>HHPMAETQTLLRNFGNVYDNPVLLDRSVTAPVTEGFNVVLASFQALYLQYQKHHFVVEGSEFYSLHEFFNESYNQVQDHIHEIGERLDGLGGVPV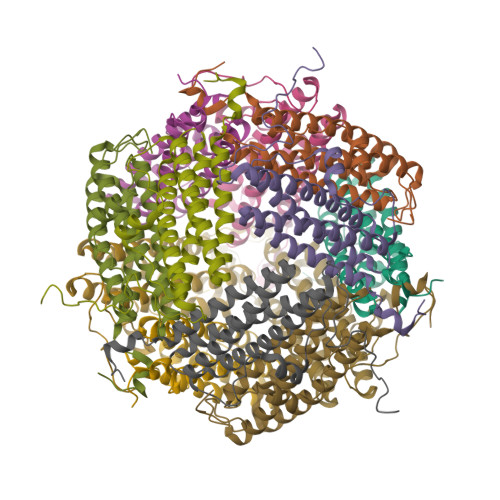ATFSKLAELTCFEQESEGVYSSRQMVENDLAAEQAIIGVIRRQAAQAESLGDRGTRYLYEKILLKTEERAYHLSHFLAKDSLTLGFVQAA[4x]>KTEQQIADIVNRTITPLMQEQAIPGMAVAVIYQGKPYYFTWGKADIANNHPVTQQTLFELGSVSKTFNGVLGGDAIARGEIKLSDPVTKYWPELTGKQWQGIRLLHLATYTAGGLPLQIPDDVRDKAALLHFYQNWQPQWTPGAKRLYANSSIGLFGALAVKPSGMSYEEAMTRRVLQPLKLAHTWITVPQNEQKDYAWGYREGKPVHVSPGQLDAEAYGVKSSVIDMARWVQANMDASHVQEKTLQQGIALAQSRYWRIGDMYQGLGWEMLNWPLKADSIINGSDSKVALAALPAVEVNPPAPAVKASWVHKTGSTGGFGSYVAFVPEKNLGIVMLANK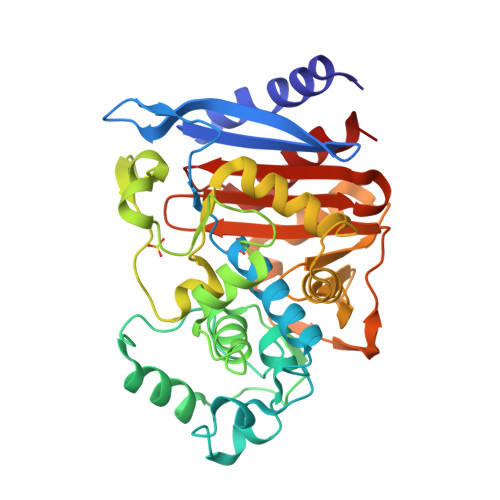SYPNPVRVEAAWRILEKLQ[4x]>GSISFHLPVNSRKCLREEIHKDLLVTGAYEITDQSGGAGGLRTHLKITDSAGHILYAKEDATKGKFAFTTEDYDMFEVCFESKGTGRIPDQLVILDMKHGVEA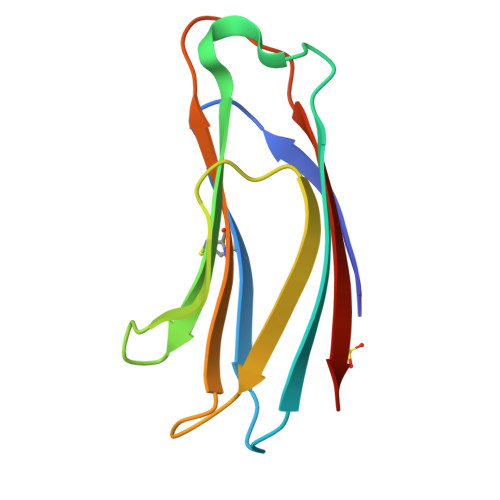[4x]> MSNKEGSGGFRKRKHDNFPHNQRREGKDVNSSSPVMLAFKSFQQELDARHDKYERLVKLSRDITVESKRTIFLLHRITSAPDMEDILTESEIKLDGVRQKIFQVAQELSGEDMHQFHRAITTGLQEYVEAVSFQHFIKTRSLISMDEINKQLIFTTEDNGKENKTPSSDAQDKQ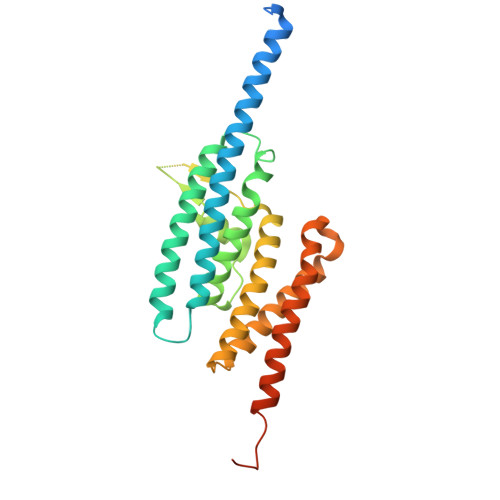FGTWRLRVTPVDYLLGVADLTGELMRMCINSVGNGDIDTPFEVSQFLRQVYDGFSFIGNTGPYEVSKKLYTLKQSLAKVENACYALKVRGSEIPKHMLADVFSVKTEMIDQEEGIS During chromosome replication, the nascent leading strand is synthesized by DNA polymerase epsilon (Pol ε), which associates with the sliding clamp processivity factor proliferating cell nuclear antigen (PCNA) to form a processive holoenzyme. For high-fidelity DNA synthesis, Pol ε relies on nucleotide selectivity and its proofreading ability to detect and excise a misincorporated nucleotide. For proofreading and mismatch excision, the 3′ end of the nascent strand must be partially melted from the template strand and guided toward the Pol ε exonuclease domain active site (exo site), which is located almost 40 Å away from the pol site. Our atomic model of human Pol ε cat closely resembles the crystal structure of the S. cerevisiae homolog, with an identical domain organization in the ‘right-hand’-shaped B-family DNA Pol fold consisting of an N-terminal domain (NTD) and the Palm, Exonuclease (Exo), Finger and Thumb domains.

To investigate how Pol ε detects and proofreads a misincorporated nucleotide, we repeated the reconstitution and structure elucidation using DNA that contained a T–C mismatch at the 3ʹ end of the nascent strand. The pol site harbors an incoming ddATP that forms a Watson–Crick base pair with the templating thymidine. Notably, we observe Pol ε only in the open conformation and extensive three-dimensional (3D) classification did not reveal any heterogeneity within the Finger domain. The absence of closed or partially closed states, despite the presence of a complementary nucleotide bound in the active site, suggests that the open conformation is favored when Pol ε is bound to a mismatch-containing substrate and may serve as a fidelity checkpoint after mismatch incorporation. The backbone of the nascent strand displays a subtle distortion at the T–C mismatch in the postinsertion site. The terminal cytosine base in the nascent strand is retracted from the templating thymidine and rotated toward the major groove. This increases the gap between the nucleobase faces and renders the base stacking with the incoming nucleotide imperfect. Most notable are the release of DNA coordination by R955 and of the interactions that Palm residues E858 and D860 form with Thumb residue K954. This rearrangement destabilizes the domain interface between Palm and Thumb, as well as the coordination of DNA near the pol site, which may serve as a trigger for subsequent conformational changes in the proofreading mechanism.

> MSLRSGGRRRADPGADGEASRDDGATSSVSALKRLERSQWTDKMDLRFGFERLKEPGEKTGWLINMHPTEILDEDKRLGSAVDYYFIQDDGSRFKVALPYKPYFYIATRKGCEREVSSFLSKKFQGKIAKVETVPKEDLDLPNHLVGLKRNYIRLSFHTVEDLVKVRKEISPAVKKNREQDHASDAYTALLSSVLQRGGVITDEEETSKKIADQLDNIVDMREYDVPYHIRLSIDLKIHVAHWYNVRYRGNAFPVEITRRDDLVERPDPVVLAFAIATTKLPLKFPDAETDQIMMISYMIDGQGYLITNREIVSEDIEDFEFTPKPEYEGPFCVFNEPDEAHLIQRWFEHVQETKPTIMVTYNGDFFDWPFVEARAAVHGLSMQQEIGFQKDSQGEYKAPQCIHMDCLRWVKRDSYLPVGSHNLKAAAKAKLGYDPVELDPEDMCRMATEQPQTLATYSVSDAVATYYLYMKYVHPFIFALCTIIPMEPDEVLRKGSGTLCEALLMVQAFHANIIFPNKQEQEFNKLTDDGHVLDSETYVGGHVEALESGVFRSDIPCRFRMNPAAFDFLLQRVEKTLRHALEEEEKVPVEQVTNFEEVCDEIKSKLASLKDVPSRIECPLIYHLDVGAMYPNIILTNRLQPSAMVDEATCAACDFNKPGANCQRKMAWQWRGEFMPASRSEYHRIQHQLESEKFPPLFPEGPARAFHELSREEQAKYEKRRLADYCRKAYKKIHITKVEERLTTICQRENSFYVDTVRAFRDRRYEFKGLHKVWKKKLSAAVEVGDAAEVKRCKNMEVLYDSLQLAHKCILNSFYGYVMRKGARWYSMEMAGIVCFTGANIITQARELIEQIGRPLELDTDGIWCVLPNSFPENFVFKTTNVKKPKVTISYPGAMLNIMVKEGFTNDQYQELAEPSSLTYVTRSENSIFFEVDGPYLAMILPASKEEGKKLKKRYAVFNEDGSLAELKGFEVKRRGELQLIKIFQSSVFEAFLKGSTLEEVYGSVAKVADYWLDVLYSKAANMPDSELFELISENRSMSRKLEDYGEQKSTSISTAKRLAEFLGDQMVKDAGLSCRYIISRKPEGSPVTERAIPLAIFQAEPTVRKHFLRKWLKSSSLQDFDIRAILDWDYYIERLGSAIQKIITIPAALQQVKNPVPRVKHPDWLHKKLLEKNDVYKQKKISELFTLEGRRQVTMAEA>MKKPRIDMHSHFFPRISEQEAAKFDANHAPWLQVSAKGDTGSIMMGKNNFRPVYQALWDPAFRIEEMDAQGVDVQVTCATPVMFGYTWEANKAAQWAERMNDFALEFAAHNPQRIKVLAQVPLQDLDLACKEASRAVAAGHLGIQIGNHLGDKDLDDA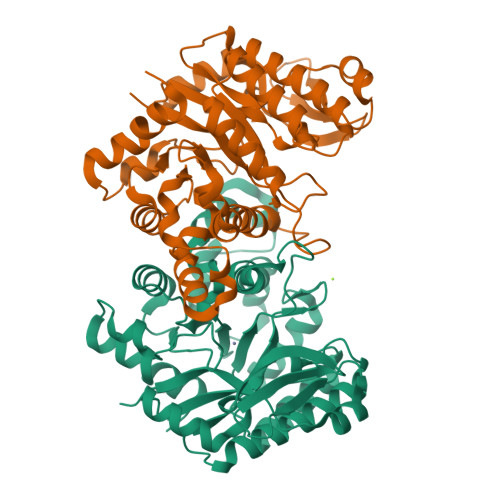TLEAFLTHCANEDIPILVHPWDMMGGQRMKKWMLPWLVAMPAETQLAILSLILSGAFERIPKSLKICFGGGGGSFAFLLGRVDNAWRHRDIVREDCPRPPSEYVDRFFVDSAVFNPGALELLVSVMGEDRVMLGSDYPFPLGEQKIGGLVLSSNLGESAKDKIISGNASKFFNINV[2x]>[2x]MRILDYDKVIERILEFIREKGNNGVVIGISGGVDSATVAYLATKALGKEKVLGLIMPYFENKDVEDAKLVAEKLGIGYKVINIKPI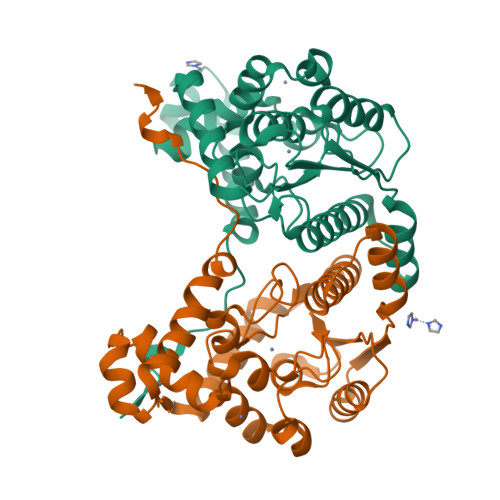VDSFVENLELNLDRKGLGNIMSRTRMIMLYAHANSLGRIVLGTSNRSEFLTGYFTKWGDGASDYAPIINLYKTEVWEIAKRIGVPERIVKKKPSAGLWEGQTDEDELGISYNLLDEILWRMIDLKIGKEEIAKDLGIPLSLVERVEELIKKSEHKRRLPIGPSFEDLIVGP> EEEWEELGSGIVPSFKERRPFHERQKDVEEIRSQQPNKVPVIIERFDGERSLPLMDRCKFLVPEHITVAELMSIVRRRLQLHPQQAFFLL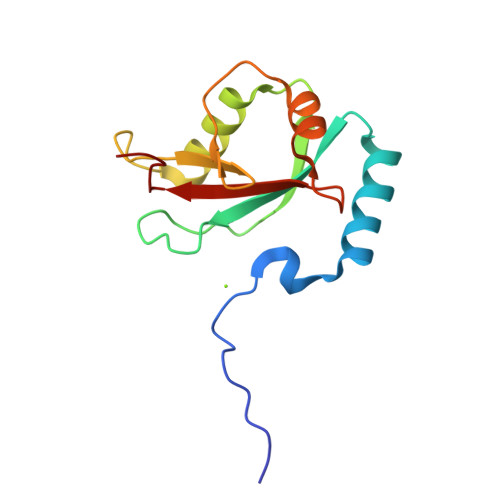VNERSMVSNSMSMSNLYSQERDPDGFVYMVYTSQPAFG> MDLLAELQWRGLVNQTTDEDGLRKLLNEERVTLYCGFDPTADSLHIGHLASILTMRRFQQAGHRPIALVGGATGLIGDPSGKKSERTLNAKETVEAWSARIKEQLGRFLDFEADGNPAKIKNNYDWIGPLDVITFLRDVGKHFSVNYMMAKESVQSRIETGISFTEFSYMMLQA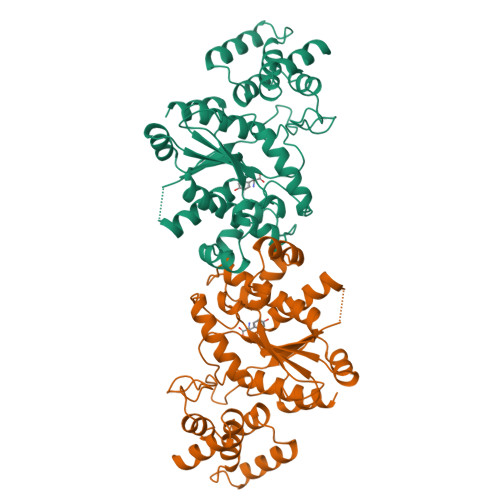YDFLRLYETEGCRLQIGGSDQWGNITAGLELIRKTKGEARAFGLTIPLVTKADGTKFGKTESGTIWLDKEKTSPYEFYQFWINTDDRDVIRYLKYFTFLSKEEIEALEQELREAPEKRAAQKTLAEEVTKLVHGEEALRQAIRIS1-(2-phenylethyl)-3,4-dihydroisoquinoline 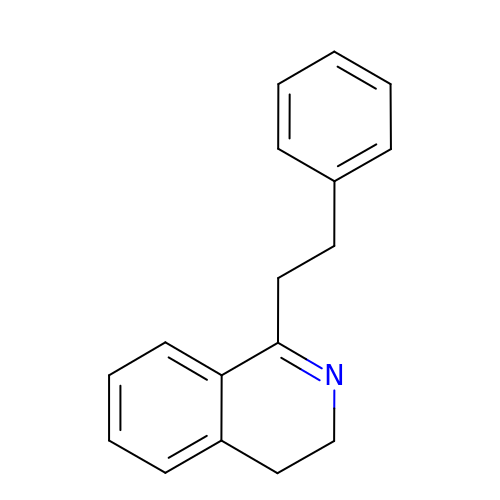| C17 H17 N | GDEYQNLNJXESFX-UHFFFAOYSA-N>[4x]MPEVLPTGKNIHALDPQAIPTAAAVQSAKVVVDRLLARQTAENNNQWPETIAMVLWGTDNI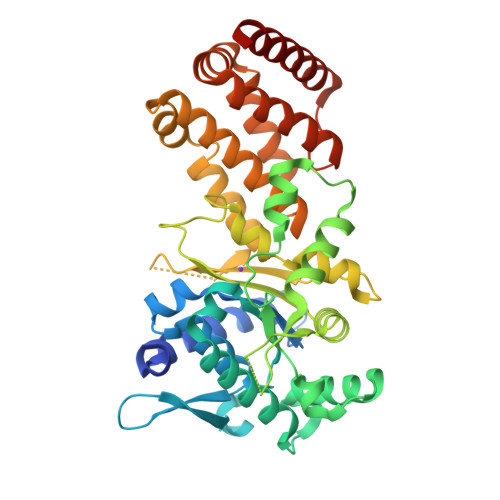KTYGESLAQVLWLVGARPLPDSLGRVNKVELIPLEELGRPRIDVVVNCSGVFRDLFINQMALIDRAIKMAAEADEPLELNFIRKHALQQASELGIDLRQAATRVFTNASGSYAANVNLAVENSSWEQESELQDMYLSRKSFAFSADSPGTMQQARELFETALKTVDVTFQNLDSSEISLTDVSHYFDSDPTKLVAALRGDGKQPKAYIADTTTANAQVRTLSETVRLDSRTKLLNPKWYEGMLAHGYEGVREISKRLVNTMGWSATAGAVDNWVYEEANATFILDEQMRQRLLNTNPHSFRKMVSTFLELHGRGYWETSEANLELLRQLYQEVEDKIEGVELEHHHHHH>[4x]MHGSNKLPGFATRAIHHGYDPQDHGGALVPPVYQTATFTFPTVEYGAACFAGEQAGHFYSRISNPTLNLLEARMASLEGGEAGLALASGMGAITSTLWTLLRPGDEVLLGNTLYGHTFAFLHHGIGEFGVKLRHVDMADLQALEAAMTPATRVIYFESPANPNMHMADIAGVAKIARKHGATVVVDNTYCTPYLQRPLELGADLVVHSATKYLSGHGDITAGIVVGSQALVDRIRLQGLKD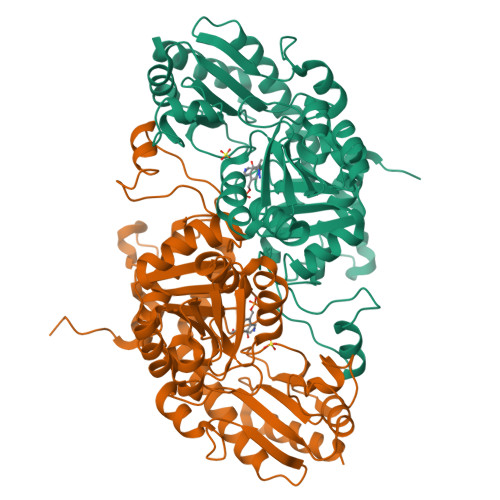MTGAVLSPHDAALLMRGIKTLNLRMDRHCANAQVLAEFLARQPQVELIHYPGLASFPQYTLARQQMSQPGGMIAFELKGGIGAGRRFMNALQLFSRAVSLGDAESLAQHPASMTHSSYTPEERAHYGISEGLVRLSVGLEDIDDLLADVQQALKASA>[2x]GMATCAVEVFGLLEDEENSRIVRVRVIAGIGLAKKDILGASDPYVRVTLYDPMNGVLTS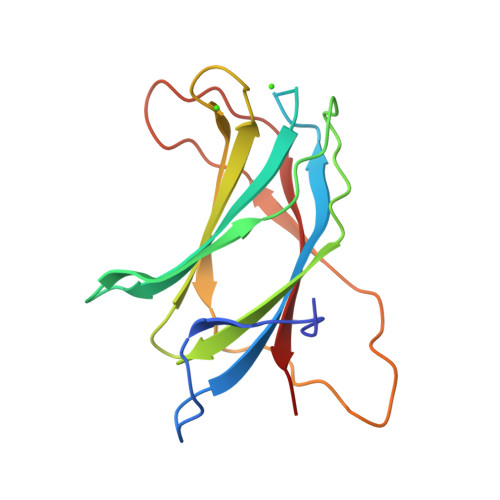VQTKTIKKSLNPKWNEEILFRVHPQQHRLLFEVFDENRLTRDDFLGQVDVPLYPLPTENPRLERPYTFKDFVLHPRSHKSRVKGYLRLKMTYLP>ALYEDPPDHKTSPSGKPATLKICSWNVDGLRAWIKKKGLDWVKEEAPDILCLQETKCSENKLPAELQELPGLSHQYWSAPSDKEGYSGVGLLSRQCPLKVSYGIGDEEHDQEGRVIVAEFDSFVLVTAYVPNAGRGLVRLEYRQRWDEAFRKFLKGLASR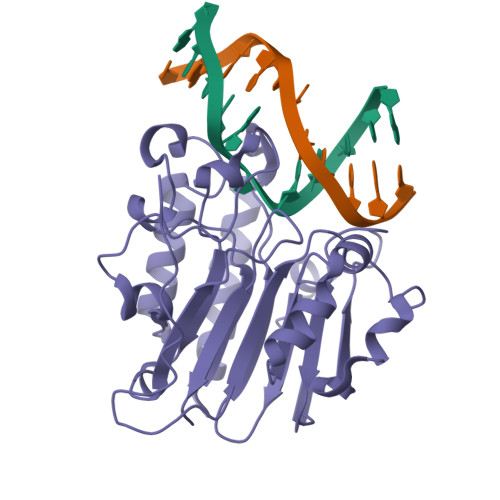KPLVLCGDLNVAHEEIDLRNPKGNKKNAGFTPQERQGFGELLQAVPLADSFRHLYPNTPYAYTFWTYMMNARSKNVGWRLDYFLLSHSLLPALCDSKIRSKALGSDHCPITLYLAL[2x]> GCCCG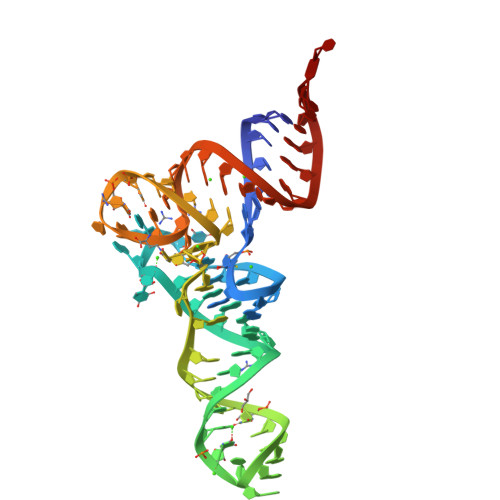GAUAGCUCAGUCGGUAGAGCAGGGGAUUGAAAAUCCCCGUGXCCUUGGUUCGAUUCCGAGUCCGGGCACCA> YPPSMDWRKKGNFVSPVKNQGSCGSCWTFSTTGALESAV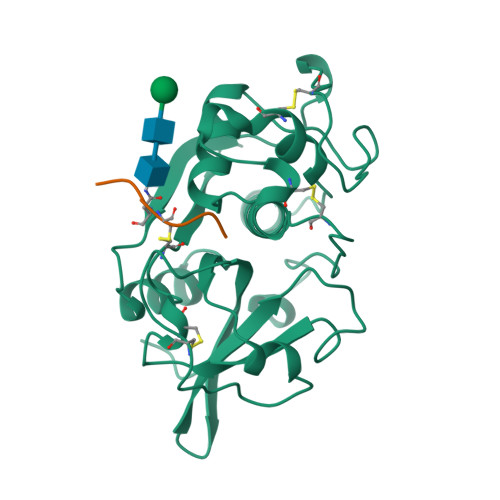AIATGKMLSLAEQQLVDCAQNFNNHGCQGGLPSQAFEYIRYNKGIMGEDTYPYKGQDDHCKFQPDKAIAFVKDVANITMNDEEAMVEAVALYNPVSFAFEVTNDFLMYRKGIYSSTSCHKTPDKVNHAVLAVGYGEENGIPYWIVKNSWGPQWGMNGYFLIERGKNMCGLAACASYPIPLV;> EPQNCSAT> SEFEAVIKVISSACKTYCGKTSPSKKEIGAMLSLLQKEGLLMSPSDLYSPGSWDPITAALSQRAMILGKSGELKTWGLVLGALK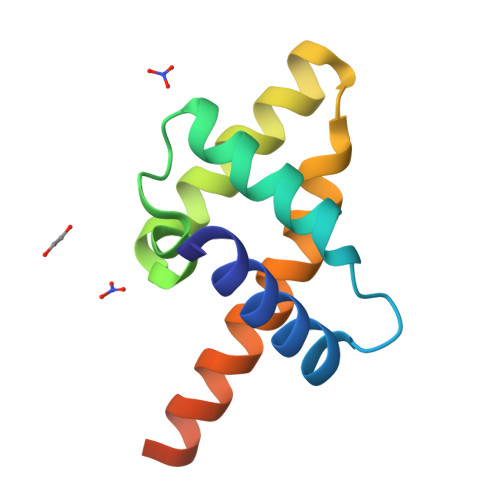AAREEQVTSEQAKFWLGLGG>[10x]MAELPPGRLATTEDYFAQQAKQAVTPDVMAQLAYMNYIDFISPFYSRGCSFEAWELKHTPQRVIKYSIAFYAYGLASVALIDPKLRALAGHDLDIAVSKMKCKRVW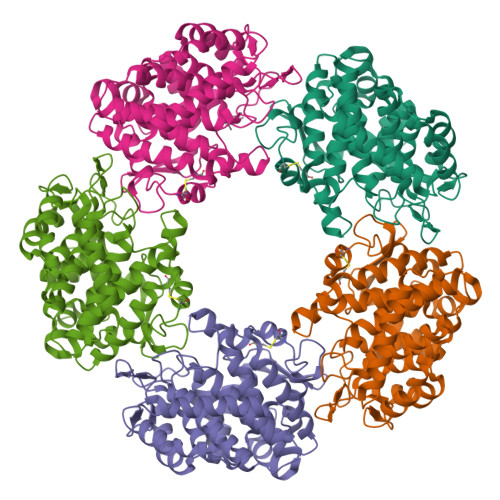GDWEEDGFGTDPIEKENIMYKGHLNLMYGLYQLVTGSRRYEAEHAHLTRIIHDEIAANPFAGIVCEPDNYFVQCNSVAYLSLWVYDRLHGTDYRAATRAWLDFIQKDLIDPERGAFYLSYHPESGAVKPWISAYTTAWTLAMVHGMDPAFSERYYPRFKQTFVEVYDEGRKARVRETAGTDDADGGVGLASAFTLLLAREMGDQQLFDQLLNHLEPPAKPSIVSASLRYEHPGSLLFDELLFLAKVHAGFGALLRMPPPAAKLAGK>[2x]SMKLTIPELSLVVLIGSSGSGKSTFAKKHFKPTEVISSNFCRGLVSDDENDQTVTGAAFDVLHYIVSKRLQLGKLTVVDATNVQESARKPLIEIAKDYHCFPVAVVFNLPEKVCQERN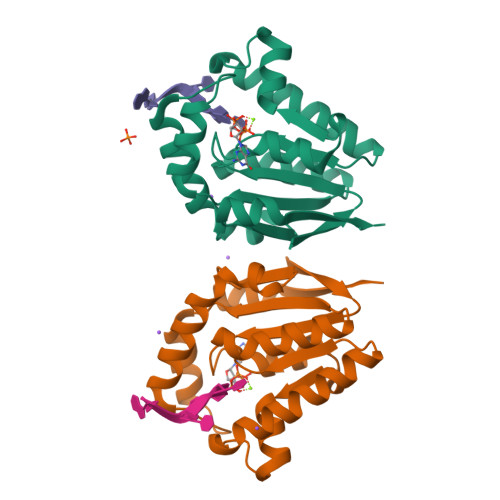KNRTDRQVEEYVIRKHTQQMKKSIKGLQREGFRYVYILNSPEEVEEVVFERQP> MSAIVGLCLLSEKVVLSRSLTDEVSKLYKLNRGNVKEPRKYATERMSTQSKPVALQVPVSTIILDYKNEDFIKQNPTYSAMDIIGSPSNTAPQTAFQSIMPSLSALFNTPFIQGAFRHRIISSMGPEISYLVMVIGPPSGFMDTPNVSSAQSSVHTVSNADVDLNDIIAINSTMAKSTKLVSASTLQAMLVNDVYDRCMDLDGILLSQALPFFRNYVNVQSKGSLPPAVAACLNTPIKELFSMGSGKREPLALEFRKDNEGQCIGIVLPKGHEGDTLSSRYPAVFINESEPFSDKERSELSELKRTDSDAYEKLYSETISKHVSDGSYGNRVIISHKMSRLSNGGVKIIGRFKISDFNTVKKNLSSRSGEIDSAKEQWEALSGNGLVTDSNISMLHDKILDTITSNKPGVVLRDGNKKSENIVVCFKNGFPNKKHSLLQLTKNGISVVSLDELTDAGILVESTGPDRVRRSPKVLANKLSSFKGR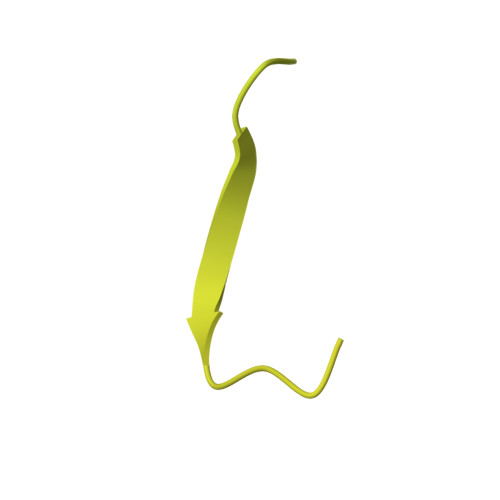KVTLDVDNMSTEALIQKLSTL tert-butyl (1-((4-(dibenzylamino)-4-oxobutyl)amino)-4-methyl-1-oxopentan-2-yl)carbamate | C29 H41 N3 O4 | 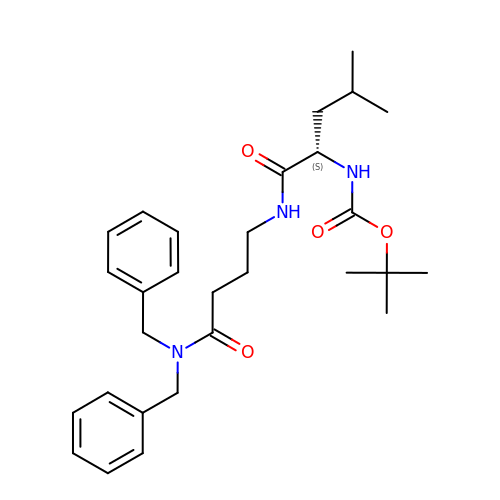RIIFVLHFONFLOV-VWLOTQADSA-N>[4x]GSDNINIPTLTLMEEVLLMGLRDREGYLSFWNDSISYALRGCIIIELALRGKIRILDDSARKRFDLSERLIEVIDSSKTGEVLLDETLQLMKNDEPLSISNWIDLLSGETWNLLKINYQLKQVRERLA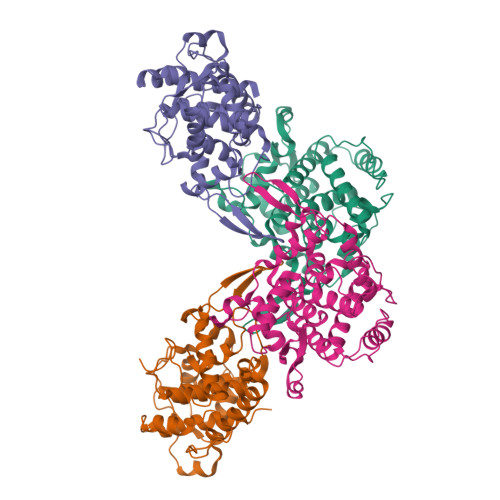KGLVDKGVLRTEMKNFFLFDMATHPIADASCKEAIKRRVLSVLVSRNMELSYNEYFPETTSFKIIRTLALICGSYGANVLENVLTTLEYEKRDKAISRAEEIMAQFSQYPFDLEKETELGVSVNLNKEVKEEIENNPGHDLQLEVIAGVFEVFSRMDMLL> NFDNPVY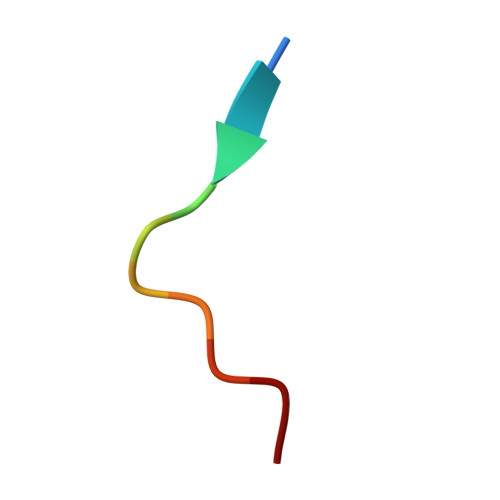RKT(5P)-3-phenyl-5-(1H-tetrazol-5-yl)-2,1-benzoxazole 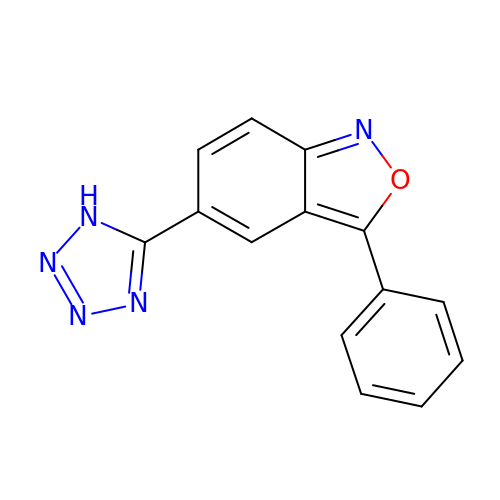| C14 H9 N5 O | QREZWQBEFHLIQN-UHFFFAOYSA-N>[8x]GSHMELTEDLNMELRVFFDTNKSNIKDQYKPEIAKVAEKLSEYPNATARIEGHTDNTGPRKLNERLSLARANSVKSALVNEYNVDASRLS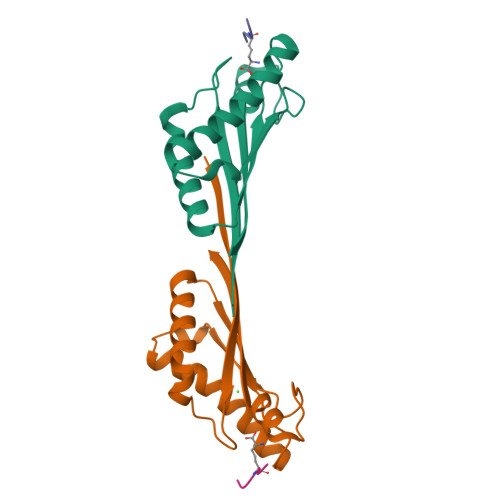TQGFAWDQPIADNKTKEGRAMNRRVFATITGSR;>[8x]AEKAA Fluorenylmethyloxycarbonyl chloride | C15 H11 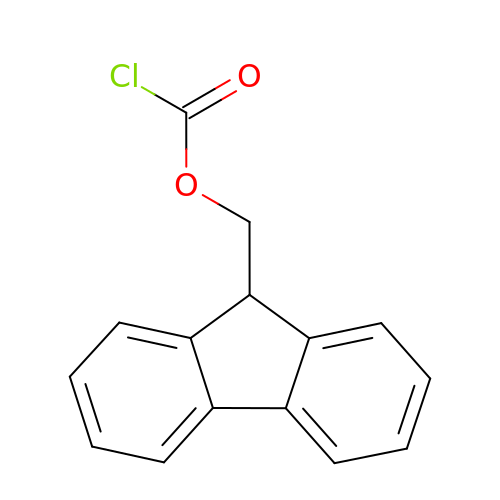Cl O2 | IRXSLJNXXZKURP-UHFFFAOYSA-N N-(5-sulfamoyl-1,3,4-thiadiazol-2-yl)cyclohexanecarboxamide 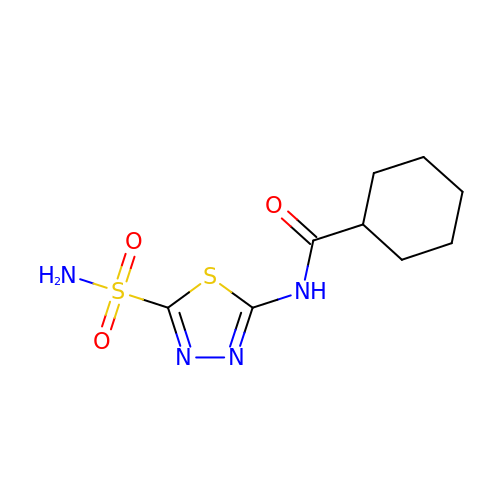| C9 H14 N4 O3 S2 | JZWSZGVTKNYBGX-UHFFFAOYSA-N DT homologs from Streptomyces albireticuli (17% identity to DT) and Seinonella peptonophila (20% identity to DT), despite showing no toxicity toward human cells, display significant structural similarities to DT sharing both the overall Y-shaped architecture of DT as well as the individual folds of each domain. Moreover, each of the individual domains preserve their respective folds: the central split β-sheet motif in the catalytic domain characteristic of the ADP-ribosyl transferase (ADPRT) superfamily; the three-layered α-helical translocation domain; and, the Ig-like jelly-roll fold in the receptor-binding domain. Additionally, both DT homologs maintain the pinched disulfide loop at the junction between the C- and T-domains. Given these structural similarities, and for purposes of clarity and simplicity, we refer to these two DT homologs hereafter as Albireti Toxin (AT) and Peptono Toxin (PT). By striking contrast, we found that AT and PT do not display any measurable toxicity on Vero cells even at µM concentrations.

Experimental phase for the DT-like protein from S. albireticuli was obtained from a 2.7 Å SAD dataset using selenomethionine (SeMet) derivatized protein crystals. Whereas the homolog from S. albireticuli (S.a) displays a Tm comparable to DT (46.5 °C cf. 48.25 °C), the homolog from S. peptonophila (S.p) is significantly more thermostable (Tm = 59.5 °C). In ATR and PTR, the 16 amino acid insertion between β9 and β10 contributes to an ~25 amino acid “lid,” hinging at ATG550 and ATN576 (PTP571 and PTD596), that folds back over and occludes the presumed receptor binding surface. Attempts to unmask a cryptic HBEGF binding site through genetic deletion of the lid in ATR proved unsuccessful, further demonstrating a lack of receptor recognition, and suggesting that the lids are not responsible for the lack of binding to HBEGF. By contrast, in AT and PT, only Y54 and E148 are absolutely conserved: in both, an Arginine is seen in place of the H21 residue; and in AT an Asparagine is seen in place of Y65. Remarkably, the T-domain of AT lacks His residues in the T domain entirely. Instead, this region (TH1-4) is stabilized by two salt-bridges between residues in TH1/TH3 and TH2/TH3.

>MTTAVENIQVAEITPSTRIVYRGVSPAEFIYLEGNKFSRAQSPTQGNDDPQWKALYTGSDANVSSRNITDNPGGVVKIEYPSDWKVLEITSTTPSQKWHNDMGEAWPVWRAVKKWAASNQVDLPDVTASNIDDYLLLDELGKKKIILKKPIGEDDVSSHEFIIPWKMAETVAQNKIDSTSDPAAKFFTPDDLDSTTKQPKDQAAVRRILKKWDAYSCKGGASATFGVASLCGINVAAYKADIEKLIKDVYEDPNFSDLKNRTGGPQKDKDTLKGYYERLKPKVETLRPLKAGVSSAVGAAGAISWAIGVADAFTSENVSSFDKAAAVTAIVPGLGECVGIANAIDKRDPEGLIINTISMAALMASAAVPVLAPIGVALDAGLAAAQGVATVLEYLEIGQPARTPLPVSSPKTHKGVTAAWVGSERIIAHRPRPGMRQHIFSVSIDSSKPEYTAPLIEVAGVRADGKLDPSPEWIRIRQNHYPIPFRFEKLSGDSPYAFRCVLLRPTTITRTEPVYVTFAYMTSDMTCRTGESDPNKACSPNNPAIAVRFGSLVKNEDERSVLAVTWPGPSIRPETNWIKLPYSIHPY[4x]>SNAMTAPRAWRPIAGGPPAGPLVLAVDFAATGRPEAAFADLVARLDPGTEVWESLQPPLGTETGMVAEDYVTRWEEEVRASGRRIGAVLGFCAGSAFAGELAVRLARSQPRSPRLVVFDPESPTTSTLYYQFRKVVESLAGVLGEQAA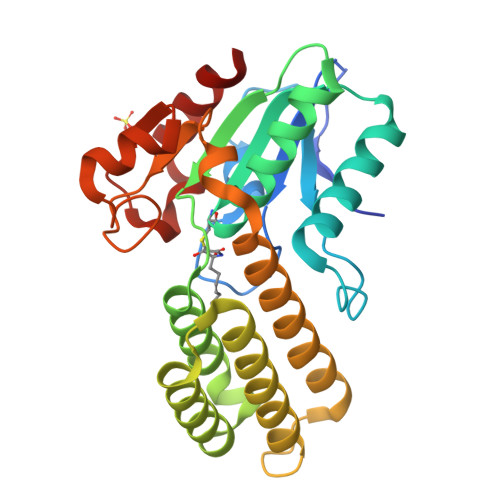REALAEGTAAADRIGDVEGLGAELVRVFTAAGRAACAAADLDDEFADELTATYRSFVSYLVAAAAVDHVKCWSGAVAVSSATPTSGLNPLDPAARAALVERELTFDVHHADLLRDPGVARAVARLLA[2x]Since DNA/RNA duplexes are known to be less stable than RNA/RNA duplexes, we have examined the impact of dA, dI, and dG substitutions on RNA structure and nonenzymatic template copying. In this study, we have investigated the effects of 2′-deoxyribo-purines on nonenzymatic template copying by conducting thermodynamic, structural, and kinetic analyses. Structural analyses of RNA duplexes containing 2′-deoxyribo-purine nucleotides suggest that the observed destabilization is likely due to reduced solvation effects, since base pairing and sugar conformations are unchanged. Our results suggest that a primordial genetic polymer containing both ribo- and 2′-deoxyribo- nucleotides would likely behave similarly to RNA but with somewhat slower template copying chemistry, offset by a possible advantage in strand separation and exchange, which could in turn facilitate cycles of replication.

Among these, four sequences (dAU1, dAU2, dAUS1, and dAUS2) contained base pairs involving deoxyadenosine (dA:U and dA:s2U), four (dGC1, dGC2, dGCS1, and dGCS2) contained deoxyguanosine base pairs (dG:C and dG:s2C), and two (dICS1 and dICS2) included base pairs with deoxyinosine (dI:s2C). In contrast, sequences containing dG:s2C formed distinct crystal lattices. Notably, the dGCS1 structure also crystallized in space group H32, but with a duplex per unit cell instead of a single strand. Notably, sequences containing dG:s2C pairs crystallized in a distinct lattice from the same sequence with G:s2C pairs, which may reflect a markedly increased flexibility in dG sugar pucker conformation compared to dA or dI. This interpretation is consistent with thermodynamic data showing a greater entropic penalty associated with replacing rG with dG. In contrast, base pairs involving deoxyguanosine (dG) display enthalpic gains but entropic penalties compared to their G-containing counterparts. The net ΔG°25°C penalty for base pairs with dG is ~0.5–0.6 kcal/mol. Although the G:s2C pair is thermodynamically less stable than A:s2U and I:s2C, the smaller ΔG° penalty associated with dG incorporation results in the dG:s2C pair exhibiting comparable stability to dA:s2U and dI:s2C.

>[2x]AGAGAAGAUCUUCUCU> MAYKRTFGHIPGHPEGSTYSNRRQVQKAGLHAHLQAGISGTAKQGADAIVLNGGYPDDRDYGDEIIYTGHGGQDPVTKKQIRDQDLDDPGNAGLVRSQLEGLPVRVIRGAGGEKPYSPSSGYRYDGLYKVVAHWFANHEDAPQFRVCQFQLVKIYDQVAAGVVVDNPDLSATAESTSVQGPAPHKKTTVSKAVRSAQVVKNVKGWHKHRCQVCGIVIEVDVGPYSQGAHIRPLGRKHGGPDVESNMLCLCPNDHVRFDNGALYITDDLKVVNALNGEVIGPLRVHPRHVIDLDHIRYHRSQLPNIPLEGSS

TagI belongs to the recently characterized SRA-HNH family of modification-dependent restriction endonucleases (REases) that also includes ScoA3IV (Sco5333) and TbiR51I (Tbis1). The SRA-HNH REases are characterized by the presence of an SRA (SET and RING finger associated) domain at the N-terminus and an HNH (histidine-asparagine-histidine) domain at the C-terminus. Our data show that TagI is a member of the NTP-independent dimeric REases that cleave DNA at a distance from the modified cytosine base. We attribute the modification specificity to the SRA domains, and the RYN/RY specificity to the HNH-domain dimer.

The crystals diffracted to 2.9 Å resolution, belonged to space group P4(1)2(1)2 and contained a single TagI protomer in the asymmetric unit. As predicted by the analysis of the amino acid sequence, TagI consists of an N-terminal SRA domain and a C-terminal HNH domain. The linker that connects the domains (residues 168–192) is not represented by electron density in the crystals, presumably due to disorder. TagI crystals contained a dimer located on a crystallographic two-fold axis and mediated by the interactions between the HNH domains. The TagI SRA domain can be described, similarly to the prototypical UHRF1 SRA domain, as a distorted β barrel, which unlike perfect β-barrels has a ‘gap’, i.e. adjacent strands that should, but do not actually engage in main chain hydrogen bonding interactions. In the case of TagI (and in UHRF1), the walls of the pocket for the flipped base are built from tyrosine residues, Tyr55 and Tyr67. The TagI HNH domain is built around the core ββα-Me motif of HNH endonucleases. The TagI HNH domain is organized around two divalent metal cations, a structural Zn2+ ion and a catalytic divalent metal ion. The identity of the latter ion in the crystal is uncertain, but we tentatively interpret it as a Na+ ion. The structural Zn2+ ion in TagI is coordinated by three cysteines, presumably in the thiolate form, and an aspartate.>[4x]Q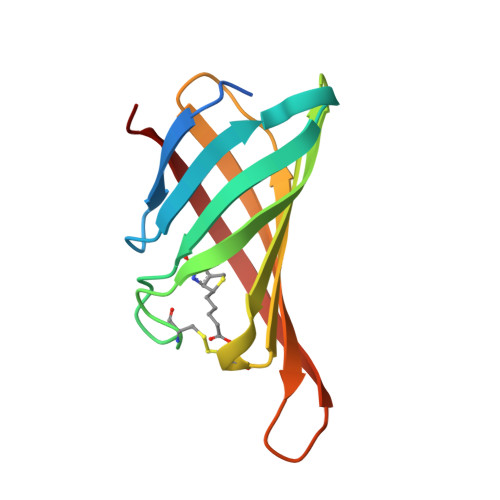TVEAMAQGLPAPSYWKNERGSELLIWSANSGTIQGTFTNHAQGFACQGIPYPAAGSVSPTGLYFVVTFAQCNSFTRWVGTIKGSQMPTSWTLFYVDNKGKPSRLKGGDIFTRVW DNMT1 is an essential enzyme that maintains genomic DNA methylation, and its function is regulated by mechanisms that are not yet fully understood. UHRF1 recognizes hemimethylated DNA via its SET and RING-associated (SRA)7–9 and catalyzes double monoubiquitination at K18 and K23 on histone H3 (H3Ub2) which, in turn, recruits DNMT1 and stimulates its enzymatic activity. Previously reported structures of apo-DNMT1 and DNMT1:DNACG/CG revealed a dual-auto-inhibitory mechanism in which the RFTS domain and the Auto-Inhibitory Linker are embedded into the catalytic core, thereby inhibiting the access of cognate DNA. Our results reveal both the large-scale displacements of inhibitory modules (RFTS, CXXC, Auto-Inhibitory Linker), as well as more detailed changes, particularly the switch by which the same hydrophobic pocket, initially bound to inhibitory phenylalanines, engages activating phenylalanines, which releases the DNA Recognition Helix and permits catalysis.

In order to understand the detailed molecular mechanism for DNMT1 activation, we have determined the cryogenic electron microscopy (cryo-EM) structure of human DNMT1 (aa:351–1616), stimulated by the H3Ub2 tail and in an intermediate complex with a hemimethylated DNA analog. The target cytosine in hemimethylated DNA was replaced by a 5-fluorocytosine (5fC) to form an irreversible covalent complex with DNMT122. 3D variability analysis by cryoSPARC23 revealed 2 types of particles: Type I particles with 2.5 Å resolution, in which the CXXC domain was ordered, and Type II particles with 2.2 Å resolution, in which the CXXC was disordered. The atomic models of DNMT1 were constructed from the two types; these structures were essentially the same (except for the CXXC domain), therefore in the rest of the paper we will focus on the Type I DNMT1 particle, with the ordered CXXC. In this structure, the RFTS domain, Auto-Inhibitory Linker, N-terminal β-sheet of BAH1 (aa:731–755), and some loops and linkers were invisible, reflecting their flexibility. The structured elements of the ternary complex showed that the catalytic core of DNMT1 bound to hemimethylated DNA, the catalytic loop (aa:1224–1238) recognized flipped-out 5fC, and the Target Recognition Domain (TRD) residues (Cys1499, Leu1500, Trp1510, Leu1513, Met1533, and Gly1534) bound to the methyl-group of 5mC. The new position of the CXXC leads to a structural deformation of the BAH1 N-terminal β-sheet and induces a different orientation of the BAH1 loop (aa:765–775) (2a center). These structural changes then lead to full eviction of the Auto-Inhibitory Linker from the catalytic core and causes the Auto-Inhibitory Linker to adopt a highly disordered structure. However, the superimposition of the CXXC:DNA complex onto the ternary complex structure revealed major steric clashes with the catalytic domain, suggesting that DNA binding by the CXXC is fully suppressed when DNMT1 is active.

> PKCIQCGQYLDDPDLKYGQHPPDAVDEPQMLTNEKLSIFDANESGFESYEALPQHKLTCFSVYCKHGHLCPIDTGLIEKNIELFFSGSAKPIYDDDPSLEGGVNGKNLGPINEWWITGFDGGEKALIGFSTSFAEYILMDPSPEYAPIFGLMQEKIYISKIVVEFLQSNSDSTYEDLINKIETTVPPSGLNLNRFTEDSLLRHAQFVVEQVESYDEAGDSDEQPIFLTPCMRDLIKLAGVTLGQRRAQARRQTIRHSTREKDRGPTKATTTKLVYQIFDTFFAEQIEKDDREDKENAFKRRRCGVCEVCQQPECGKCKACKDMVKFGGSGRSKQACQERRCPNMAMKEADDDEEVDDNIPEMPSPKKMHQGKKKKQNKNRISWVGEAVKTDGKKSYYKKVCIDAETLEVGDCVSVIPDDSSKPLYLARVTALWEDSSNGQMFHAHWFCAGTDTVLGATSDPLELFLVDECEDMQLSYIHSKVKVIYKAPSENWAMEGGMDPESLLEGDDGKTYFYQLWYDQDYARFESPPKTQPTEDNKFKFCVSCARLAEMRQKEIPRVLEQLEDLDSRVLYYSATKNGILYRVGDGVYLPPEAFTFNIKLSSPVKRPRKEPVDEDLYPEHYRKYSDYIKGSNLDAPEPYRIGRIKEIFCPKKSNGRPNETDIKIRVNKFYRPENTHKSTPASYHADINLLYWSDEEAVVDFKAVQGRCTVEYGEDLPECVQVYSMGGPNRFYFLEAYNAKSKSFEDPPNHARSPGNKGKGKGKGKGKPKSQACEPSEPEIEIKLPKLRTLDVFSGCGGLSEGFHQAGISDTLWAIEMWDPAAQAFRLNNPGSTVFTEDCNILLKLVMAGETTNSRGQRLPQKGDVEMLCGGPPCQGFSGMNRFNSRTYSKFKNSLVVSFLSYCDYYRPRFFLLENVRNFVSFKRSMVLKLTLRCLVRMGYQCTFGVLQAGQYGVAQTRRRAIILAAAPGEKLPLFPEPLHVFAPRACQLSVVVDDKKFVSNITRLSSGPFRTITVRDTMSDLPEVRNGASALEISYNGEPQSWFQRQLRGAQYQPILRDHICKDMSALVAARMRHIPLAPGSDWRDLPNIEVRLSDGTMARKLRYTHHDRKNGRSSSGALRGVCSCVEAGKACDPAARQFNTLIPWCLPHTGNRHNHWAGLYGRLEWDGFFSTTVTNPEPMGKQGRVLHPEQHRVVSVRECARSQGFPDTYRLFGNILDKHRQVGNAVPPPLAKAIGLEIKLCMLAKARESASAKIKEEEAAKD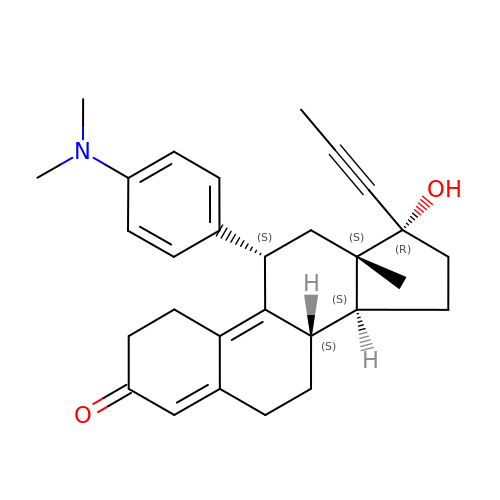11-(4-DIMETHYLAMINO-PHENYL)-17-HYDROXY-13-METHYL-17-PROP-1-YNYL-1,2,6,7,8,11,12,13,14,15,16,17-DODEC AHYDRO-CYCLOPENTA[A]PHENANTHREN-3-ONE | C29 H35 N O2 | VKHAHZOOUSRJNA-GCNJZUOMSA-N>MAHHHHHHMIDLTGKTSLITGASSGIGSAIARLLHKLGSKVIISGSNEEKLKSLGNALKDNYTIEVCNLANKEECSNLISKTSNLDILVCNAGITSDTLAIRMKDQDFDKVIDINLKANFILNREAIKKMIQKRYGRIINISSIVGIAGNPGQANYCASKAGLIGMTKSLSYEVATRGITVNAVAPGFIKSDM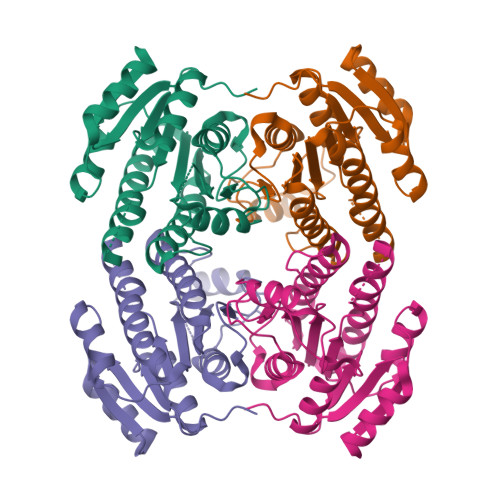TDKLNEKQREAIVQKIPLGTYGIPEDVAYAVAFLASNNASYITGQTLHVNGGMLMV[2x]> MSDIFDEAASFRSYQSKLGRDGRASAATATLTTKIRIFVPATNSPELRWELTLFALDVIRSPSAAESMKIGAAFTLISMYSERPGALIRSLLNDPDIEAVIIDVGSMLNGIPVMERRGDKAQEEMEGLMRILKTARESSKGKTPFVDSRAYGLRITDMSTLVSAVITIEAQIWILIAKAVTAPDTAEESETRRWAKYVQQKRVNPFFALTQQWLTEMRNLLSQSLSVRKFMVEILMEVKKGGSAKGRAVEIISDIGNYVEETGMAGFFATIRFGLETRYPALALNEFQSDLNTIKGLMLLYREIGPRAPYMVLLEESIQTKFAPGGYPLLWSFAMGVATTIDRSMGALNINRGYLEPMYFRLGQKSARHHAGGIDQNMANKLGLNSDQVAELAAAVQETSVGRQDNNMQAREAKFAAGGVLVGGGEQDID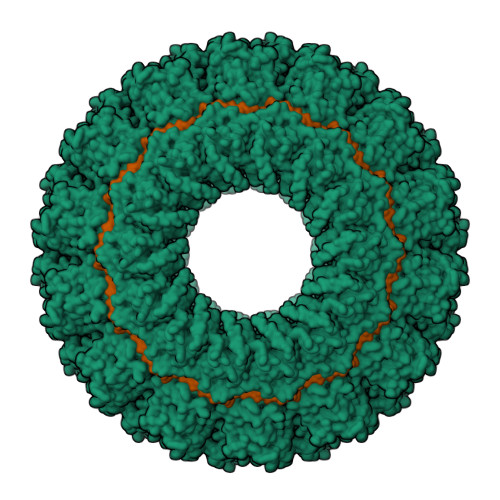EEEEPIEHSGRQSVTFKREMSMSSLADSVPSSSVSTSGGTRLTNSLLNLRSRLAAKAIKESTAQSSSERNPPNNRPQADSGRKDDQEPKPAQNDLDFVRADV> GAQVSTQKTGAHETGLRASGNSIIHYTNINYYKDAASNSANRQDFTQDPGKFTEPV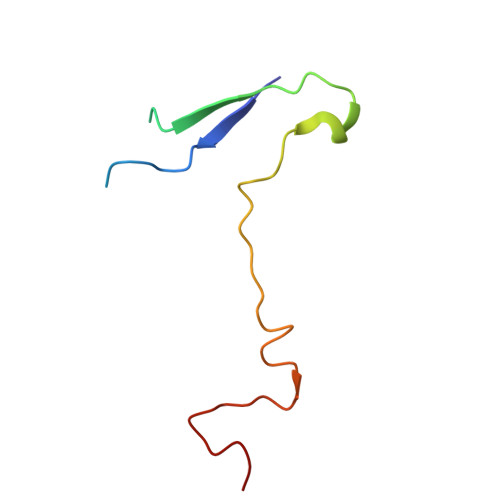KDIMVKSLPALN>[4x]GPGSMAAATFHWDDPLLLDQQLADDERMVRDAAHAYAQGKLAPRVTEAFRHETTDAAIFREMGEIGLLGPTIPEQYGGPGLDYVSYGLIAREVERVDSGYRSMMSVQSSLVMVPIFEFGSDAQKEKYLPKLATGEWI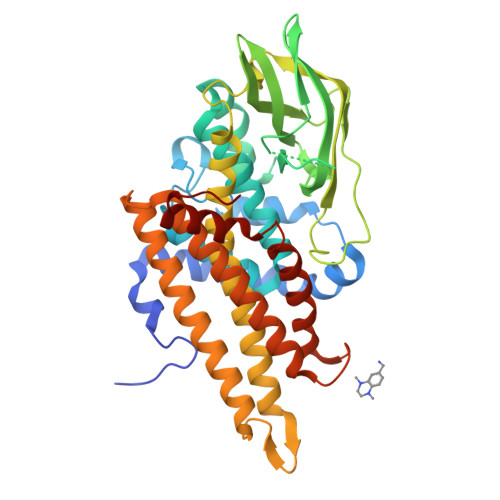GCFGLTEPNHGSDPGSMVTRARKVPGGYSLSGSKMWITNSPIADVFVVWAKLDEDGRDEIRGFILEKGCKGLSAPAIHGKVGLRASITGEIVLDEAFVPEENILPHVKGLRGPFTCLNSARYGIAWGALGAAESCWHIARQYVLDRKQFGRPLAANQLIQKKLADMQTEITLGLQGVLRLGRMKDEGTAAVEITSIMKRNSCGKALDIARLARDMLGGNGISDEFGVARHLVNLEVVNTYEGTHDIHALILGRAQTGIQAFF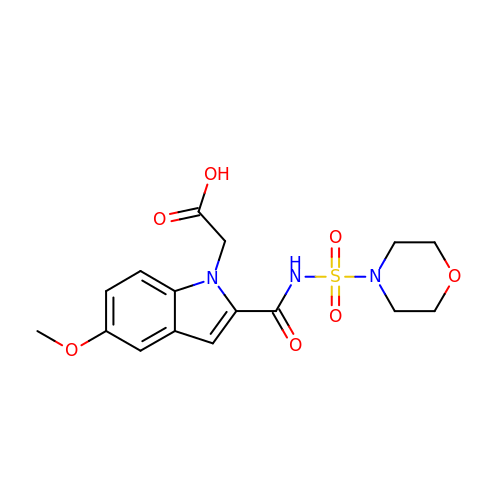{5-methoxy-2-[(morpholin-4-ylsulfonyl)carbamoyl]-1H-indol-1-yl}acetic acid | C16 H19 N3 O7 S | BNCOTZAAIISTRX-UHFFFAOYSA-N>LSCGQRLRKSLSSMTRVVGGLVALRGAHPYIAALYWGHSFCAGSLIAPCWVLTAAHCLQDRPAPEDLTVVLGQERRNHSCEPCQTL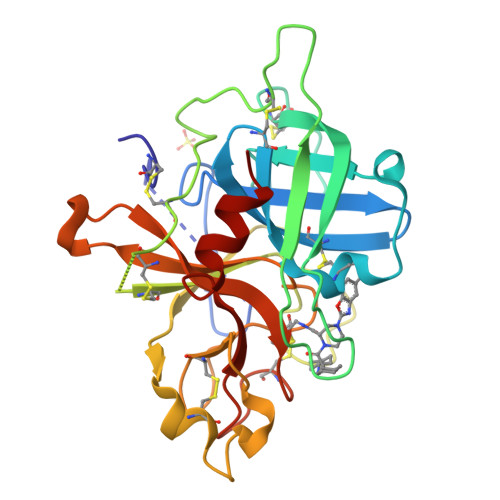AVRSYRLHEAFSPVSYQHDLALLRLQEDADGSCALLSPYVQPVCLPSGAARPSETTLCQVAGWGHQFEGAEEYASFLQEAQVPFLSLERCSAPDVHGSSILPGMLCAGFLEGGTDACQGDSGGPLVCEDQAAERRLTLQGIISWGSGCGDRNKPGVYTDVAYYLAWIREHTVS[3x]> CAGCATGCCTGATACCGCA;> TGCGGTATCACCACGA;> TGCGCTGTGGCATGC;> TCGTGG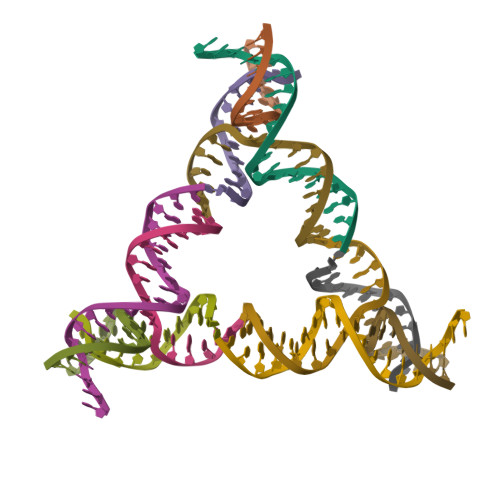ACAGCG> NG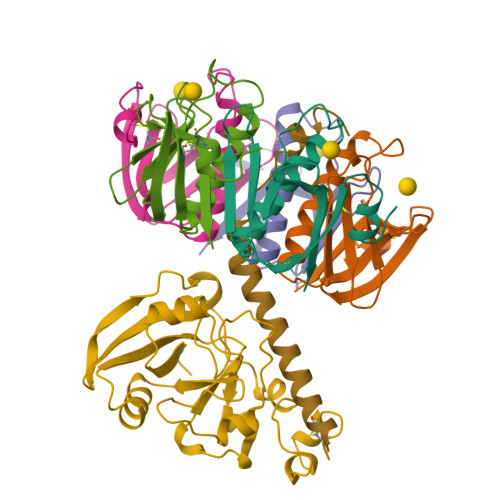DRLYRADSRPPDEIKRSGGLMPRGHNEYFDRGTQMNINLYDHARGTQTGFVRYDDGYVSTSLSLRSAHLAGQSILSGYSTYYIYVIATAPNMFNVNDVLGVYSPHPYEQEVSALGGIPYSQIYGWYRVNFGVIDERLHRNREYRDRYYRNLNIAPAEDGYRLAGFPPDHQAWREEPWIHHAPQGCG;> RTITGDTCNEETQNLSTIYLREYQSKVKRQIFSDYQSEVDIYNRIRDEL;>APQTITELCSEYRNTQIYTINDKILSYTESMAGKREMVIITFKSGETFQVEVPGSQHIDSQKKAIERMKDTLRITYLTETKIDKLCVWNNKTPNSIAAISMKN[5x]>[2x]MNPAAEAEFNILLATDSYKVTHYKQYPPNTSKVYSYFECREKKTENSKLRKVKYEETVFYGLQYILNKYLKGKVVTKEKIQEAKDVYKEHFQDDVFNEKGWNYILEKYDGHLPIEIKAVPEGFVIPRGNVLFTVENTDPECYWLTNWIETILVQSWYPITVATNSREQKKILAKYLLETSGNLDGL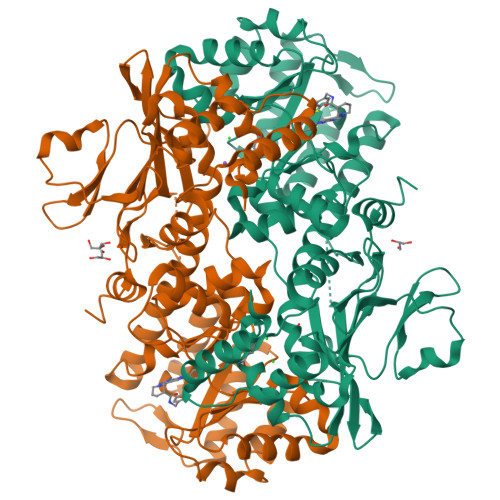EYKLHDFGYRGVSSQETAGIGASAHLVNFKGTDTVAGLALIKKYYGTKDPVPGYSVPAAEHSTITAWGKDHEKDAFEHIVTQFSSVPVSVVSDSYDIYNACEKIWGEDLRHLIVSRSTQAPLIIRPDSGNPLDTVLKVLEILGKKFPVTENSKGYKLLPPYLRVIQGDGVDINTLQEIVEGMKQKMWSIENIAFGSGGGLLQKLTRDLLNCSFKCSYVVTNGLGINVFKDPVADPNKRSKKGRLSLHRTPAGNFVTLEEGKGDLEEYGQDLLHTVFKNGKVTKSYSFDEIRKNAQLNIELEAAHHLEHHHHHH>ETLVRPKPLLLKLLKSVGAQKDTYTMKEVLFYLGQYIMTKRLYDEKQQHIVYCSNDLLGDLFGVPSFSVKEHRKIYT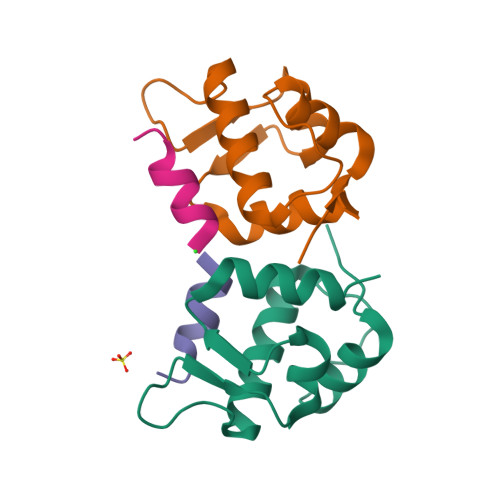MIYRNLVV[3x];>TNWYANLEKLLR[3x]>[4x]MEGERKNNNKRWYFTREQLENSPSRRFGVDPDKELSYRQQAANLLQDMGQRLNVSQLTINTAIVYMHRFYMIQSFTRFPGNSVAPAALFLAAKVEEQPKKLEHVIKVAHTCLHPQESLPDTRSEAYLQQVQDLVILESIILQTLGFELTIDHPHTHVVKCTQLVRASKDLAQTSYFMAT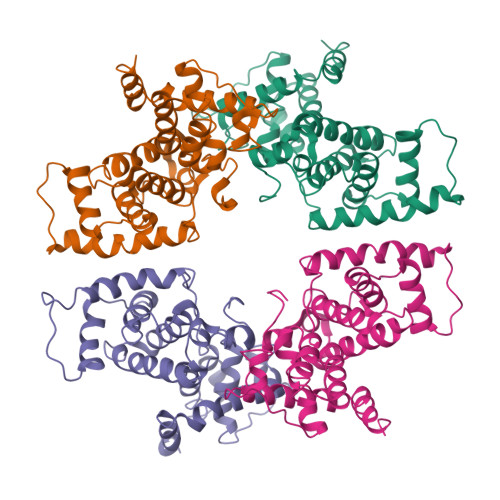NSLHLTTFSLQYTPPVVACVCIHLACKWSNWEIPVSTDGKHWWEYVDATVTLELLDELTHEFLQILEKTPNRLKRIWNWRACEAAKKTKADDRGTDEKTSEQGGTGGGSGGGSGGGSGGGTSGGVPGQNTGGQEARPNYHCQLCFLRSLGIDYLDASLRKKNKQRLKAIQQGRQPQYLL> TTPLVHVASVEKGRSYEDFQKVYNAIALKLRE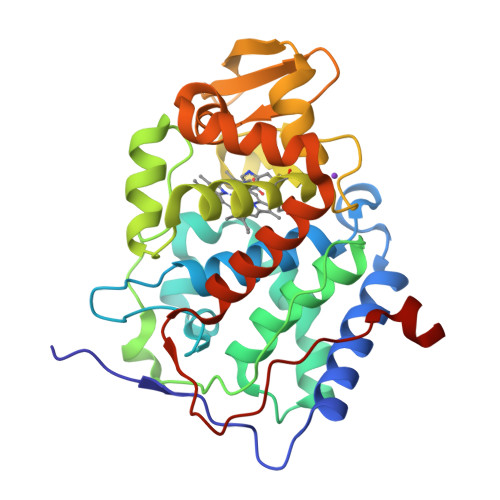DDEYDNYIGYGPVLVRLAWHTSGTWDKHDNTGGSYGGTYRFKKEFNDPSNAGLQNGFKFLEPIHKEFPWISSGDLFSLGGVTAVQEMQGPKIPWRCGRVDTPEDTTPDNGRLPDADKDADYVRTFFQRLNMNDREVVALMGAHTLGKTHLKNSGYEGPWTANPNVFDNSFYLNLLNEDWKLEKNDANNEQWDSKSGYMMLPTDYSLIQDPKYLSIVKEYANDQDKFFKDFSKAFEKLLENGITFPKDAPSPFIFKTLEEQGL> GPGQKECDNALRQLETVRELLENPVQPINDMSYFGCLDSVMENSKVLGEAMTGISQNAKNGNLPEFGDAIATASKALCGFTEAAAQAAYLVGVSDPNSQAGQQGLVEPTQFARANQAIQMACQSLGEPGCTQAQVLSAATIVAKHTSALCNSCRLASARTANPTAKRQ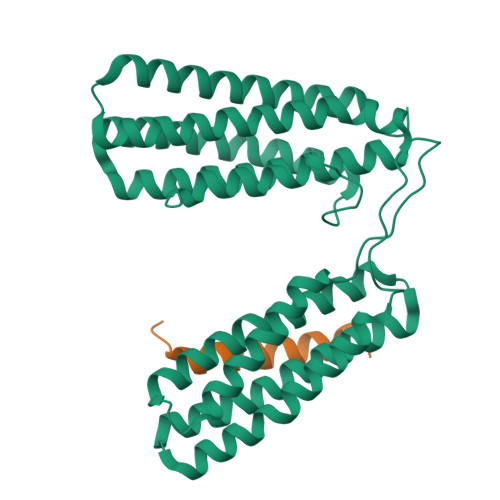FVQSAKEVANSTANLVKTIKALDGDFTEENRAQCRAATAPLLEAVDNLSAFASNPEFSSVPAQISPEGRAAMEPIVISAKTMLESAGGLIQTARALAVNPRDPPRWSVLAGHSRTVSDSIKKLITSMRDKAPGQL;> STKHILDDISTMFDALADQLDAMLD N-[N'-BENZYLOXYCARBONYL-PHENYLALANINYL]-3-AMINO-5-PHENYL-PENTANE-1-SULFONIC ACID PHENYL ESTER | C34 H36 N2 O6 S | 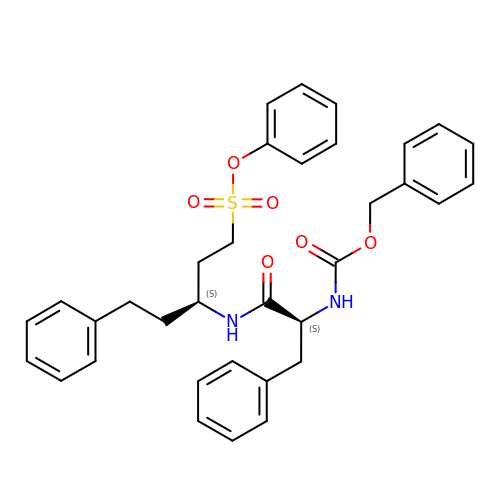SUGQHICXCRBQOI-CDZUIXILSA-N2-[(E)-(1-methylquinolin-4(1H)-ylidene)methyl]-3-(2-oxopropyl)-1,3-benzothiazol-3-ium 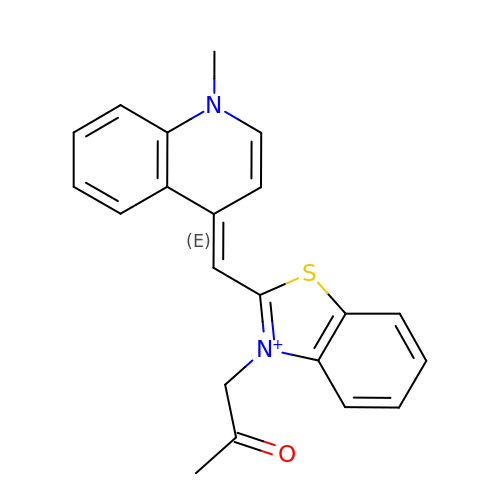| C21 H19 N2 O S | MNJLWFGXGDINRC-UHFFFAOYSA-N>[4x]SMQFTGKNVLITGASKGIGAEIARTLASMGLKVWINYRSNAEVADALKNELEEKGYKAAVIKFDAASESDFV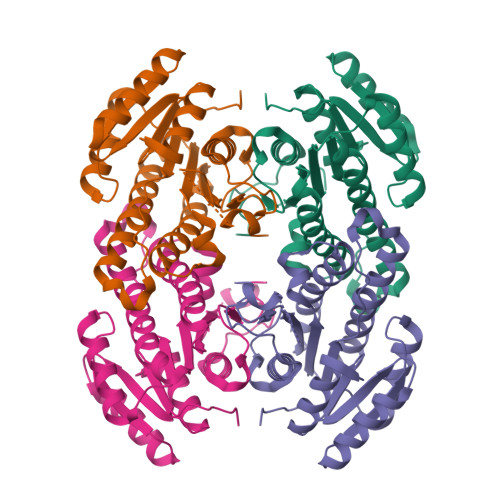EAIQAIVQSDGGLSYLVNNAGVVRDKLAIKMKTEDFHHVIDNNLTSAFIGCREALKVMSKSRFGSVVNIASIIGERGNMGQTNYSASKGGMIAMSKSFAYEGALRNIRFNSVTPGFIETDMNANLKDELKADYVKNIPLNRLGAAKEVAEAVAFLLSDHSSYITGETLKVNGGLYM>MAHHHHHHMNRLQGKRALVTGGSRGIGAAIAKRLAADGADVAITYEKSAERAQAVVAGIEALGRRAIAIQADSADPVAVRNAVDRVAEAFGGLDILVNNAGIFRAGSLDDLTLDDIDATLNVNVRAVIVASQAAARHLGEGGRIVSTGSCLATRVPDAGMSLYAASKAALIGWTQGLARDLGP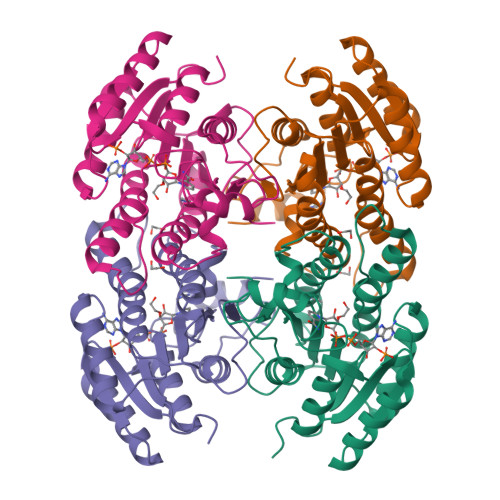RGITVNIVHPGSTDTDMNPADGAHADAQRSRMAIQQYGKADDVAALVAFVVGPEGRSINGTGLTIDGGANA[4x]> MARENEMDENLE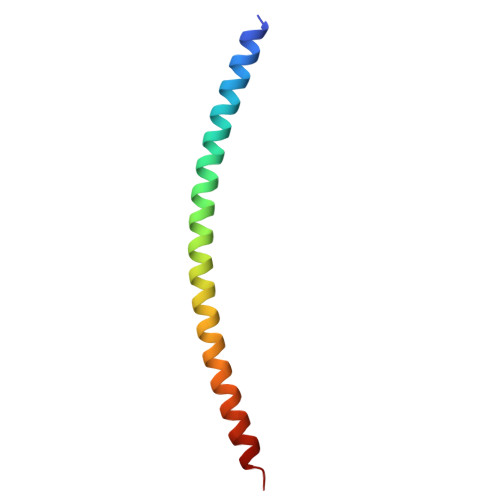QVSGIIGNLRHMALDMGNEIDTQNRQIDRIMEKADSNKTRIDEANQRATKMLG> MTDTATTPQTTDAPAFPSNRSCPYQLPDGYA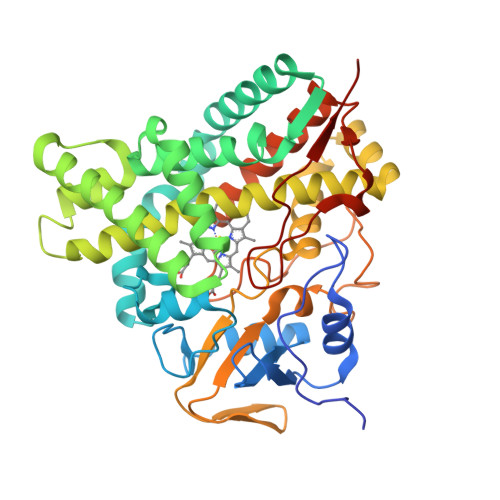QLRDTPGPLHRVTLYDGRQAWVVTKHEAARKLLGDPRLSSNRTDDNFPATSPFFEAVRESPQAFIGLDPPEHGTRRRMTISEFTVKRIKGMRPEVEEVVHGFLDEMLAAGPTADLVSQFALPVPSMVICRLLGVPYADHEFFQDASKRLVQSTDAQSALTARNDLAGYLDGLITQFQTEPGAGLVGALVADQLANGEIDREELISTAMLLLIAGHETTASMTSLSVITLLDHPEQYAALRADRSLVPGAVEELLRYLAIADIAGGRVATADIEVEGQLIRAGEGVIVVNSIANRDGTVYEDPDALDIHRSARHHLAFGFGVHQCLGQNLARLELEVILNALMDRVPTLRLAVPVEQLVLRPGTTIQGVNELPVTWHHHHHH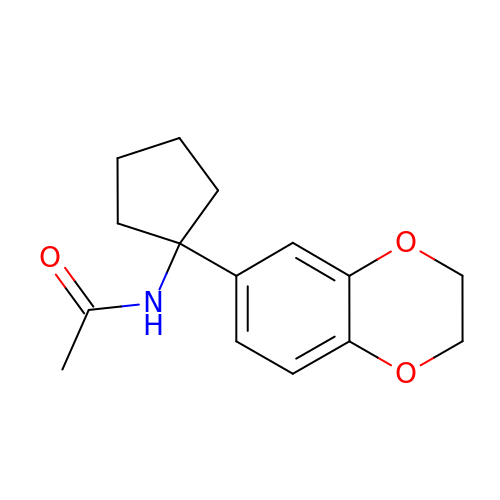N-[1-(2,3-dihydro-1,4-benzodioxin-6-yl)cyclopentyl]acetamide | C15 H19 N O3 | RVYUUTVAMYXICP-UHFFFAOYSA-N> IVG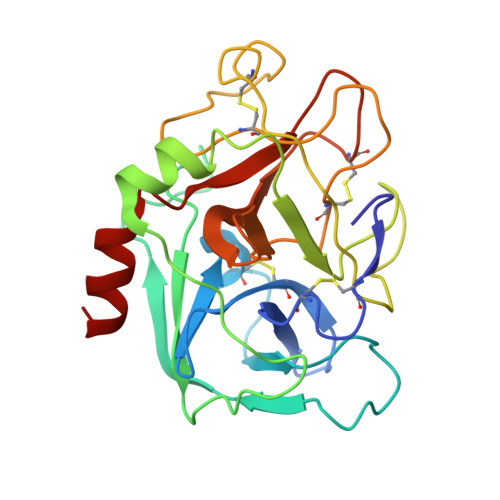GQECKDGECPWQALLINEENEGFCGGTILSEFYILTAAHCLYQAKRFKVRVGDRNTEQEEGGEAVHEVEVVIKHNRFTKETYDFDIAVLRLKTPITFRMNVAPACLPERDWAESTLMTQKTGIVSGFGRTHEKGRQSTRLKMLEVPYVDRNSCKLSSSFIITQNMFCAGYDTKQEDACQGDSGGPHVTRFKDTYFVTGIVSWGEGCARKGKYGIYTKVTAFLKWIDRSMKTR> DRVETLVFDGAKTEARAIASDIAGSVGELAAAARTMSGVLGRGHAGQSTDRAGAINLLKANLEQHGFAFGSWFAEEPKAYDGKDVIDNTERGGNADGAFTPYWSKDRNGNIQLSTFKADYAAEWYGLAAKSGKGAIT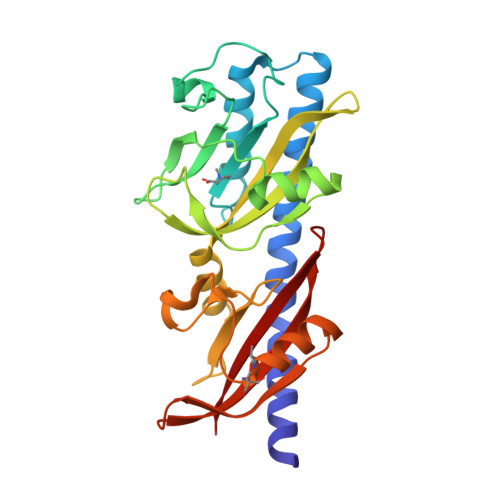QPYLAEGTDVPTTMTSIAYPVMSNGRMIGVSGVDISLAALADRLSAVKPFGSGRVYLLSQSGKWLAAPIPELLMKEYDGEGVESVKDALSTGTPRMIENLTYDGNEPFDRVVYPFSLPDVNAQWLVLVDVPR> MYSVLKQSIRPRLLATHNQFRTMITAQAVLYTQHGEPKDVLFTQSFEIDDDNLAPNEVIVKTLGSPVNPS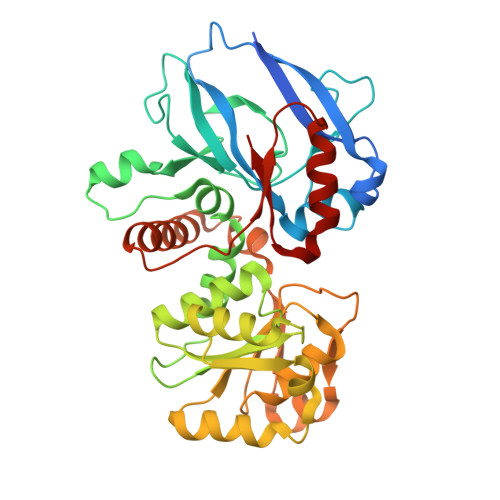DINQIQGVYPSKPAKTTGFGTTEPAAPCGNEGLFEVIKVGSNVSSLEAGDWVIPSHVNFGTWRTHALGNDDDFIKLPNPAQSKANGKPNGLTINQGATISVNPLTAYLMLTHYVKLTPGKDWFIQNGGTSAVGKYASQIGKLLNFNSISVIRDRPNLDEVVASLKELGATQVITEDQNNSREFGPTIKEWIKQSGGEAKLALNCVGGKSSTGIARKLNNNGLMLTYGGMSFQPVTIPTSLYIFKNFTSAGFWVTELLKNNKELKTSTLNQIIAWYEEGKLTDAKSIETLYDGTKPLHELYQDGVANSKDGKQLITY> AKRYWNANLDTYHPKNVSQNR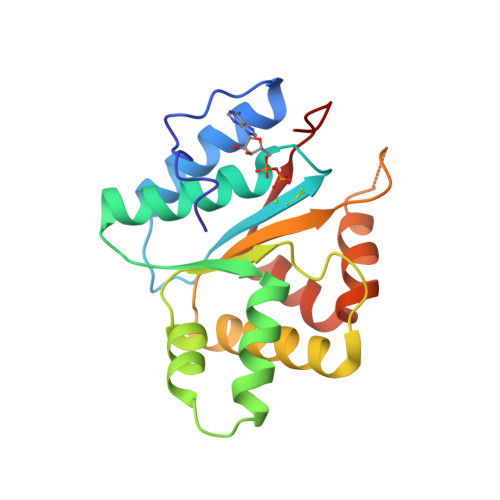ALLTIRVFVHNFNPEEGKGLTFVGSPGVGKTHLAVATLKAIYEKKGIRGYFFDTKDLIFRLKHLMDEGKDTKFLKTVLNSPVLVLDDLGSERLSDWQRELISYIITYRYNNLKSTIITTNYSLQREEESSVRISADLASRLGENVVSKIYEMNELLVIKGSDLR>GHMAIATINPTTGEICQRFKALTPAEIDAKLAKAQEAFQAYRRTSFSQRRQWLENAAAILERDTSKFAEIMTTEMGKTHQSAIAEAEKSALVCRYYAEHGEQFLANEYTETQATESYVCYQPLGILLAVMPWNFPFWQVFRFAAPALMAGNVAVLKHASNVPQCALAVEAILEAAGFPEGVFQTLLIGASQVEQVIKDPRVKAATLTGSEPAGASLASLAGQEIKPTLLELGGSDPFVVFPSADLDEAVEVGTVARTMNNGQSCIAAKRFILHEAIAAEFLEKLHLKFASLKIGDPMAPETDIGPLATEGILQDISRQVDQAVAAGAKILLGGRPLDRAGYFYPPT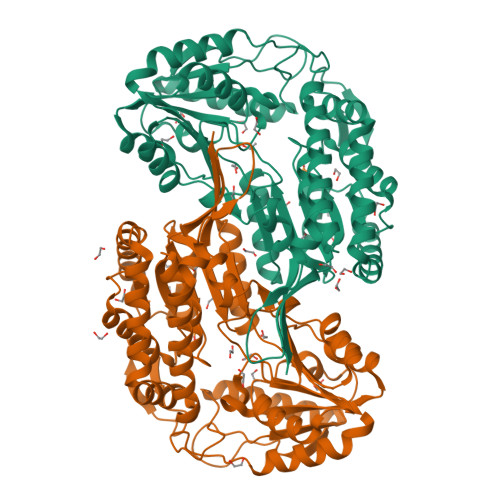ILTEIPPGAKILQEELFAPVAMVFTVKDLDQAIALANDIPFGLGASAWTNDPAEQQRFIQELDAGAVFINGMVKSDPRLPFGGTKRSGYGRELGLAGIRTFVNAKTVWLK[2x]4-[(2S,3S)-2-ethyl-3-hydroxy-5-oxopyrrolidin-1-yl]-2-(trifluoromethyl)benzonitrile | C14 H13 F3 N2 O2 | 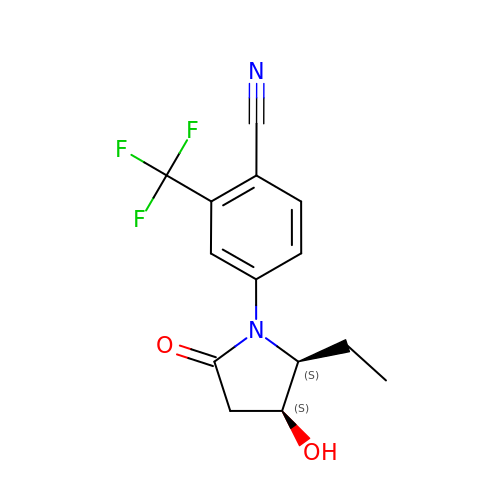LJQBTMVNFWIQQC-RYUDHWBXSA-N>SASKRAIDANQIVNRMSLDEKLGQMLMPDFRNWQKEGESSPQALTKMNDEVASLVKKYQFGGIILFAENVKTTKQTVQLTDDYQKASPKIPLMLSIDQEGGIVTRLGEGTNFPGNMALGAARSRINAYQTGSIIGKELSALGINTDFSPVVDINNNPDNPVIGVRSFSSNRELTSRLGLYTMKGLQRQDIASALKHFPGHGDTDVDSHYGLPLVSHGQERLREVELYPFQKAIDAGADMVMTAHVQFPAFDDTTYKSKLDGSDILVPATLSKKVMTGLLRQEMGFNGVIVTNALNMKAIADHFGQEEAVVMAVKAGVDIALMPASVTSLKEEQKFARVIQALKEAVKNGDIPEQQINNSVERIISLKIKRGMYPARNSDSTKEKIAKAKKIVGSKQHLKAEKKLAEKAVTVLKNEQHTLPFKPKKGSRILIVAPYEEQTASIEQTIHDLIKRKKIKPVSLSKMNFASQVFKTEHEKQVKEADYIITGSYVVKNDPVVNDGVIDDTISDSSKWATVFPRAVMKAALQHNKPFVLMSLRNPYDAANFEEAKALIAV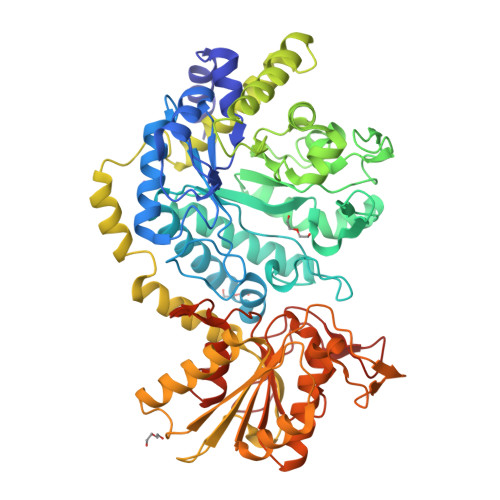YGFKGYANGRYLQPNIPAGVMAIFGQAKPKGTLPVDIPSVTKPGNTLYPLGYGLNIKTGRPL[4x]>[4x]MACPLEKALDVMVSTFHKYSGKEGDK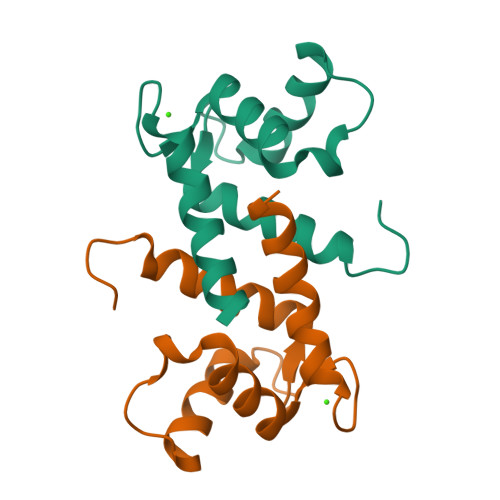FKLNKSELKELLTRELPSFLGKRTDEAAFQKLMSNLDSNRDNEVDFQEYCVFLSCIAMMCNEFFEGF> MGLPSGASIVPLAQEHIPALRRINSLLLPVAYPDSFYHKALDPLASGLFSRAILWQDTNADPPKVVGGLICRLEPNPFLSVTGEPTPVQLPADQPQRAPQAPKDTPFHAIYIQSLALLSPYRSLGLAAAALDHIIA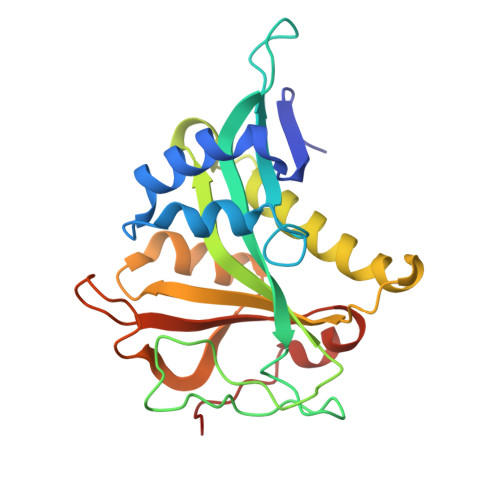TAAVLPAAGSNIDARTIYAHVWTENEEGLKWYESRGFVKEGGEPVKGYYFKLRPDTAWIVRRHIGESAKLNDVVHHHHHH> MNDIAHNLAQVRDKISAAATRCGRSPEEITLLAVSKTKPASAIAEAIDAGQRQFGENYVQEGVDKIRHFQELGVTGLEWHFIGPLQSNKSRLVAEHFDWCHTIDRLRIATRLNDQRPAELPPLNVLIQINISDENSASGIQLAELDELAAAVAELPRLRLRGLMAIPAPESEYVRQFEVARQMAVAFAGLKTRYPHIDTLSLGMSDDMEAAIAAGSTMVRIGTAIFGARDYSKK

The pyridoxal 5′‐phosphate (PLP) homeostasis protein (PLPHP) is a ubiquitous member of the COG0325 family with apparently no catalytic activity. Although the actual cellular role of this protein is unknown, it has been observed that mutations of the PLPHP encoding gene affect the activity of PLP‐dependent enzymes, B6 vitamers and amino acid levels. Here we report a detailed characterization of the Escherichia coli ortholog of PLPHP (YggS) with respect to its PLP binding and transfer properties, stability, and structure. YggS binds PLP very tightly and is able to slowly transfer it to a model PLP‐dependent enzyme, serine hydroxymethyltransferase.

We serendipitously discovered that the K36A variant of YggS, affecting the lysine residue that binds PLP at the active site, is able to bind PLP covalently. This observation led us to recognize that a number of lysine residues, located at the entrance of the active site, can replace Lys36 in its PLP binding role.> MAATAAEAVASGSGEPREEAGALGPAWDESQLRSYSFPTRPIPRLSQSDPRAEELIENEEPVVLTDTNLVYPALKWDLEYLQENIGNGDFSVYSASTHKFLYYDEKKMANFQNFKPRSNREEMKFHEFVE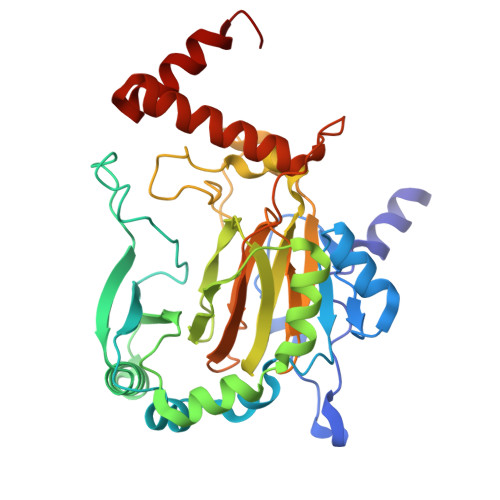KLQDIQQRGGEERLYLQQTLNDTVGRKIVMDFLGFNWNWINKQQGKRGWGQLTSNLLLIGMEGNVTPAHYDEQQNFFAQIKGYKRCILFPPDQFECLYPYPVHHPCDRHSQVDFDNPDYERFPNFQNVVGYETVVGPGDVLYIPMYWWHHIESLLNGGITITVNFWYKGAPTPKRIEYPLKAHQKVAIMRNIEKMLGEALGNPQEVGPLLNTMIKGRYN> ACPEDWGASSRTSLCFKLYAKGKHEKKTWFESRDFCRALGGDLASINNKEEQQTIWRLITASGSYHKLFWLGLTYGSPSEGFTWSDGSPVSYENWAYGEPNNYQNVEYCGELKGDPTMSWNDINCEHLNNWICQI

The human mannose receptor expressed on macrophages and hepatic endothelial cells scavenges released lysosomal enzymes, glycopeptide fragments of collagen, and pathogenic microorganisms and thus reduces damage following tissue injury. The receptor binds mannose, fucose, or N-acetylglucosamine (GlcNAc) residues on these targets. C-type carbohydrate-recognition domain 4 (CRD4) of the receptor contains the site for Ca2+-dependent interaction with sugars. The mechanisms of binding to monosaccharides and oligosaccharide substructures present in many of these ligands were examined in multiple crystal structures of CRD4.

The binding of α-methyl mannose to CRD4 is revealed by four independent copies of this complex observed in three different crystal forms: two copies of the CRD in form αMeMan/1 and one copy of the CRD in αMeMan/2 and αMeMan/3. Each structure shows the same orientation of the bound sugar. Binding of mannose residues to CRD4 results primarily from interaction of the equatorial 3- and 4-OH groups with a conserved principal Ca2+ common to almost all sugar-binding C-type CRDs. As in other C-type CRDs, the main determinants of monosaccharide binding to CRD4 are a conserved principal Ca2+ and four of the five amino acid residues that surround it. The presence of glutamic acid and asparagine residues at positions 725 and 727 in CRD4 determines specificity for mannose, GlcNAc, and other sugars with equatorial 3- and 4-OH groups. In addition to the Ca2+ ligands, the side chain of Tyr729 makes van der Waals contacts with the bound sugar. The position of the aromatic ring of Tyr729 is established in part by interactions with the side chain of Gln730. The protrusion of the tyrosine and adjacent glutamine residue creates a barrier adjacent to the sugar residue. The importance of the interaction of the sugar with Tyr729 was demonstrated by changing this residue to alanine, which caused a fivefold loss in affinity for α-methyl mannose. Mutagenesis demonstrated that these changes in the spectrum were caused by the ring current effect from the side chain of Tyr729. These results are consistent with the orientation of mannose in the primary binding site seen in the αMe-Man crystals, which places C5 and C6 above the tyrosine ring.> GSHMVKVLLALTSYNETFYSDGKKT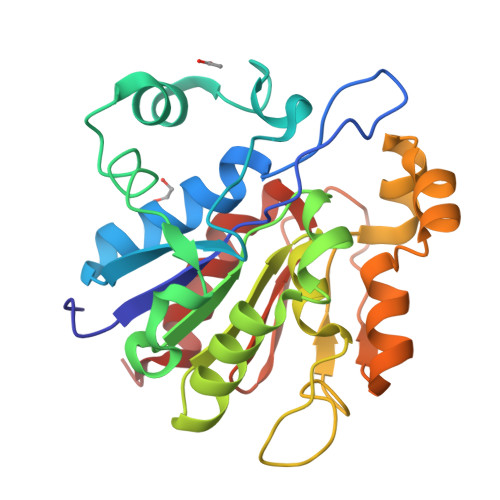GVFVVEALHPFEVFRKKGYEIQLASETGTFGWDDHSVVPDFLNGEDKEIFDNVNSEFNVALKNLKKASDLDPNDYDIFFGSAGHGTLFDYPNAKDLQKIATTVYDKGGVVSAVCHGPAIFENLNDPKTGEPLIKGKKITGFTDIGEDILGVTDIMKKGNLLTIKQVAEKEGATYIEPEGPWDNFTVTDGRIVTGVNPQSAVKTAEDVIAAFECN Sterol 14α-demethylases (CYP51s) represent a very special P450 family, regarded as a possible evolutionary progenitor for all currently existing P450s. CYP51 enzymes are found in all kingdoms of life, catalyzing the same complex, three-step stereo- and regio-specific reaction that is essential for the biosynthesis of sterols, such as cholesterol in humans and other vertebrates, and ergosterol in pathogenic fungi and protozoa, whose CYP51 orthologs are targets for azole drugs. In metazoans CYP51 is critical for the biosynthesis of sterols including cholesterol. Binding of physiological substrates, however, causes a conserved conformational switch that involves closing of the active site entrance (bordered by helices A’, F’’ and the tip of the β4 hairpin).

Here we report the first crystal structure of a non-mammalian vertebrate CYP51, from the abyssal grenadier (Coryphaenoides armatus), a deep-sea fish common in most oceans of the world at depths between one and five kilometers. Statistical analyses of the catalytic domains show 80% identity between C. armatus and human CYP51s (90% similarity). The structural similarities that we find distinguishing for both ligand-free vertebrate CYP51s include the “broken I-helix” (residues 311–313), and the “heme bulge” segment (residues 441–450) shifted away from the P450 heme. The shifted heme bulge segment in the ligand-free C. armatus and human CYP51 structures is accompanied by the loss of the conserved heme-supporting salt bridge between the imidazole nitrogen of H447 and the carboxylate oxygen of the porphyrin ring D propionate. There are, however, two striking differences between the fish and human CYP51 structures, and those are in the location of the β4 hairpin (residues 481–494) and, even more so, in the location of the FG arm (residues 232–258). The middle portion of the FG arm in the fish enzyme lacks the characteristic F’’ helix. Instead, this region of the molecule adopts a loop-like conformation and is immersed deep inside the active site pocket, approaching helix I (SRS4), strand β1–4 (SRS5), and “clashing” with the β4 hairpin (SRS6) in the superimposed human CYP51 structure. In turn, the C. armatus CYP51 β4 hairpin is moved outward, away from the active site, protruding above the surface of the protein globule. The distance between the C. armatus P242 and the corresponding proline (ending the F” helix in the human structure) is 24 Å, and the tips of their β4 hairpins (I488) are 16 Å apart (inset). Instead, it is a transient, low-populated conformation common to all CYP51s, which becomes more populated due to the placement of the high-pressure adapted enzyme at ambient conditions.

>[2x]MAKKTKCPPYIPSRIPFLGHAVAFGKNPIEFLEKAYEKYGPVVSFTMVGKTFTFLLGSDAAALMFNSKNEDLSAEDVYSKITTPVFGKGVAYDVPNPIFLEQKKMLKTGLNIAQFKKHVPIIEQETEEYIKRWGDSGETNLFVAMSELIILTASSCLHGKEIRSLLNEKVAQLYCDLDGGFSHEAWLLPSWLPLPSFRRRDRAHREIKNMFYTAIQKRRTSNEKVDDFLQTLIDATYKDGHSLSDDEIAGLLIGLLLAGQHTSSTTSSWMSFFLARDKQLQERCLAEQKAVCGEDLPPLDFDQLKELSLLDRCLKETLRLRPPIMTMMRMARSPQCVAGYTIPVGHQVCVSPTVNQRLPDSWTERDEFNPDRYLTDNAATGEKFAYVPFGAGRHRCIGEGFAYVQLKTILSTLIRKFEFDLVDGYFPTINFTTMIHTPNNPVIRYRSRT> TKAETSIGVFYVSEYGYSDRLAQAIINGITKTGVGVDVVDLGAAVD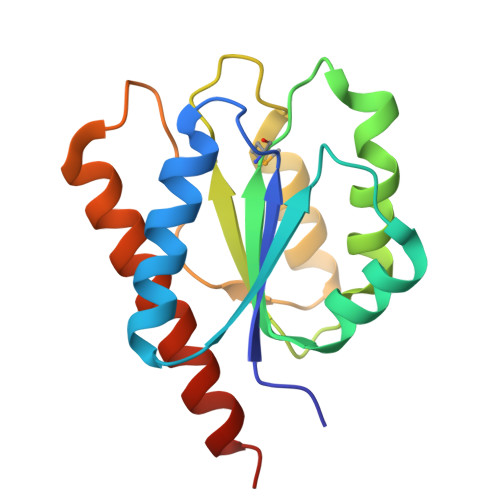LQELRELVGRCTGLVIGMSPAASAASIQGALSTILGSVNEKQAVGIFETGGGDDEPIDPLLSKFRNLGLTTAFPAIRIKQTPTENTYKLCEEAGTDLGQWVTRDRLEHHHHHH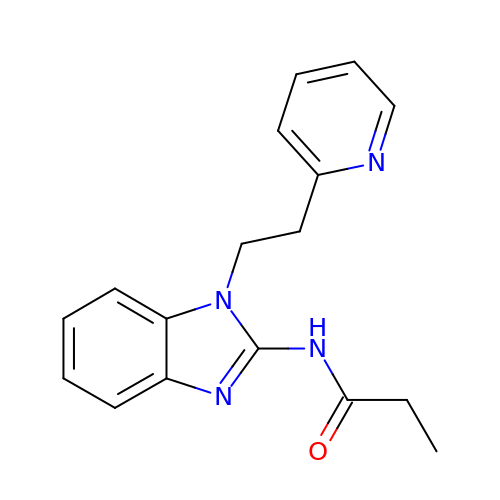~{N}-[1-(2-pyridin-2-ylethyl)benzimidazol-2-yl]propanamide | C17 H18 N4 O | XNCNQSNDNANIRM-UHFFFAOYSA-N> GSHMNQMSKISVTVNGRRYPWPRVPAIAVCLDGCEPAYLDAAIDAGLMPALKRIKERGAVRLAHSVIPSFANPNNLSIATGSPPAVHGICGNYLYEPSTGEEVMMNDPKFLRAPTIFQAFYDAGARVAVVTAKDKLRALLGKGLRFDEGRAVCFSSEKSDKATRAEHGIDNASAWLGRPVPEVYSAALSEFVFAAGVKLLREFRPDIMYLTTTDYVQHKYAPGVPEANSFYEMFDRYLAELDGLGAAIVVTADHGMKPKHKADGSPDVIYVQDLLDEWLGKDAARVILPITDPYVVHHGALGSFATAYLPDGCDRSEIMARLKAIQGVDVVLGREEACRRFELPEDRIGDIVLVSSENKTLGTSEHRHDLAALDEPLRSHGGLTEQEVPFIVNRVLPELPNAPRLRNFDAFFYAVTAAAEAG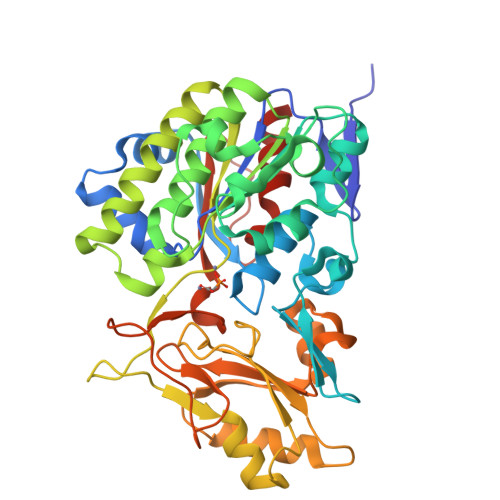AEGGL>[12x]MPSGYGVLLATHDDDTVDVFTSGRKMRLTCSPNIDAASLKKGQTVRLNEALTVVEAGTFEAVGEISTLREILADGHRALVVGHADEERVVWLADPLIAEDLPDGLPEALN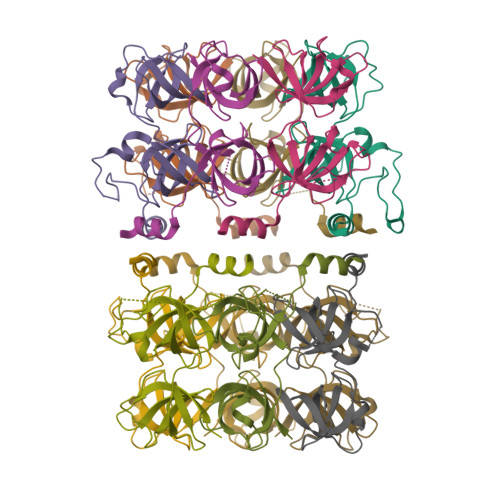DDTRPRKLRPGDSLLVDTKAGYAFERIPKAEVEDLVLEELVPR> ATYHLEDNWVGSAFLSTFTHEAIADPTHGRVNYVDQATALAKNLTYASGDTLILRADHTTTLSPSGPGRNSVRIRS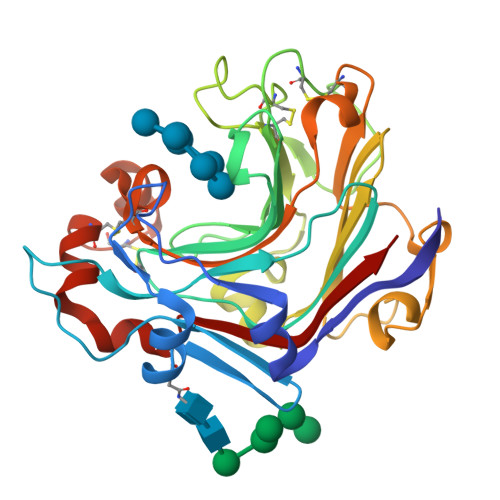IKTYTTHVAVFDVRHMPQGCGTWPAAWETDEGDWPNGGSVDIIEGVNDQSPNAMTLHTGANCAMPASRTMTGHATNNNCDVNTDGNTGCGVQAPTANSYGPSFNANGGGWYAMERTNSFIKVWFFPRNAGNVPNDIASGPATINTDNWGTPTAFFPNTNCDIGSHFDANNIIINLTFCGDWAGQASIFNGAGCPGSCVDYVNNNPSAFANAYWDIASVRVYQ> MQQIDLNVTCRYAGVFHVEKNGRYSISRTEAADLCQAFNSTLPTMDQMKLALSKGFETCRYGFIEGN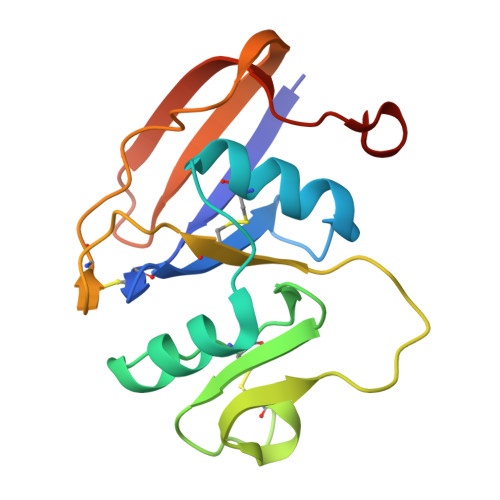VVIPRIHPNAICAANHTGVYILVTSNTSHYDTYCFNASAPPEEDCTSVTDLPNSFDGPVTITIVNRDGTRYSKKGEYRTHQEDIDAS> MSSIDNDSDVDLTEDLAVAKIVKENPVARKMVRYILSRGESQNSIITRNKLQSVIHEAAREENIAKPSFSKMFMDINAILYNVYGFELQGLPSKNNMNAGGNGSNSNTNKSMPEPLGHRAQKFILLNNVPHSKNFDDFKILQSAHTYEELIVTGEYIGDDIASGTSNTLESKLSTDRDLVYKGVLSVILCIVFFSKNNILHQELIKFLETFGIPSDGSKIAILNITIEDLIKSLEKREYIVRLEEKSDT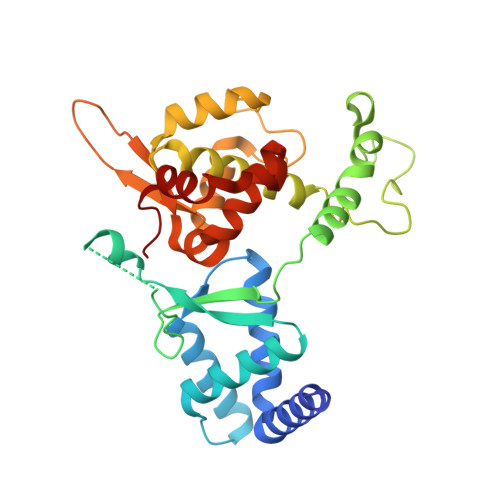DGEVISYRIGRRTQAELGLESLEKLVQEIMGLEKEQTKSLHDDIIKSIGDSYSI>MVRIIVKNVSKVFKKGKVVALDNVNINIE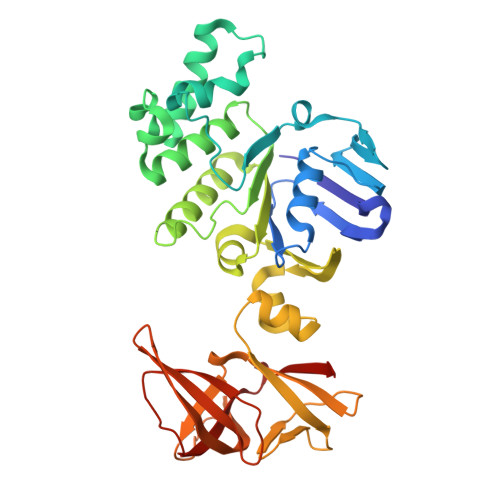NGERFGILGPSGAGKTTFMRIIAGLDVPSTGELYFDDRLVASNGKLIVPPEDRKIGMVFQTWALYPNLTAFENIAFPLTNMKMSKEEIRKRVEEVAKILDIHHVLNHFPRELSGGQQQRVALARALVKDPSLLLLDEPFSNLDARMRDSARALVKEVQSRLGVTLLVVSHDPADIFAIADRVGVLVKGKLVQVGKPEDLYDNPVSIQVASLIGEINELEGKVTNEGVVIGSLRFPVSVSSDRAIIGIRPEDVKLSKDVIKDDSWILVGKGKVKVIGYQGGLFRITITPLDSEEEIFTYSDHPIHSGEEVLVYVRKDKIKVFEKN[3x]> MKEFGDSLSLEILQIIKESQQQHGLRHGDFQRYRGYCSRRQRRLRKTLNFKMGNRHKFTGKKVTEELLTDNRYLLLVLMDAERAWSYAMQLKQEANTEPRKRFHLLSRLRKAVKHAEELERLCESNRVDAKTKLEAQAYTAYLSGMLRFEHQEWKAAIEAFNKCKTIYEKLASAFTEEQAVLYNQRVEEISPNIRYCAYNIGDQSAINELMQMRLRSGGTEGLLAEKLEALITQTRAKQAATMSEVEWRGRTVPVKIDKVRIFLLGLADNEAAIVQAESEETKERLFESMLSECRDAIQVVREELKPDQKQRDYILEGEPGKVSNLQYLHSYLTYIKLSTAIKRNENMAKGLQRALLQQQPEDDSKRSPRPQDLIRLYDIILQNLVELL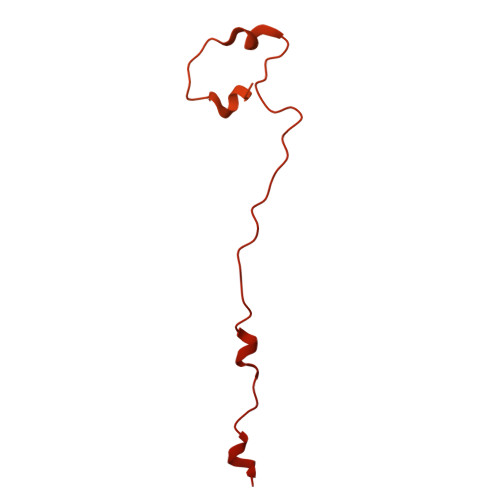QLPGLEEDKAFQKEIGLKTLVFKAYRCFFIAQSYVLVKKWSEALVLYDRVLKYANEVNSDAGAFKNSLKDLPDVQELITQVRSEKCSLQAAAILDANDAHQTETSSSQVKDNKPLVERFETFCLDPSLVTKQANLVHFPPGFQPIPCKPLFFDLALNHVAFPPLEDKLEQKTKSGLTGYIKGIFGFRS(6-phenoxy-1-benzofuran-3-yl)acetic acid | C16 H12 O4 | 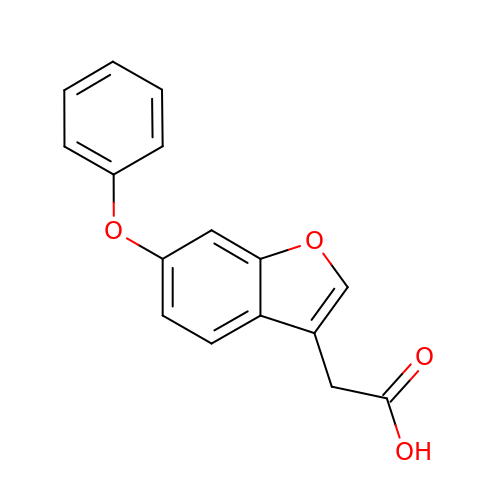SLCAFBFROXEZHX-UHFFFAOYSA-N> MAKRIATVSQTLRIGYVSSLLYGLLPEIIYLFRQQNPEIHIELIE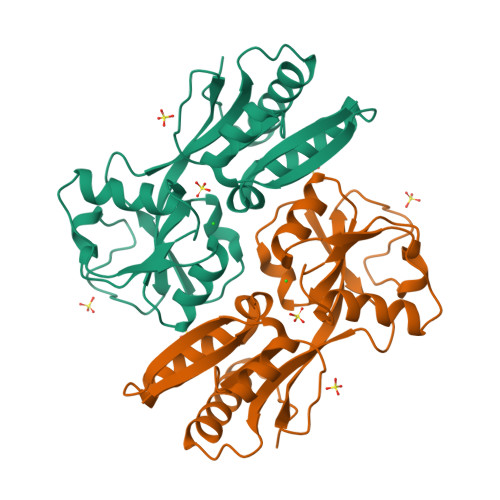CGTKDQINALKQGKIDLGFGRLKITDPAIRRIVLHKEQLKLAIHKHHHPNQFAATGVHLSQIIDEPMLLYPVSQKPNFATFIQSLFTELGLVPSKLTEIREIQLALGLVAAGEGVCIVPASAMDIGVKNLLYIPILDDDAYSPISLAVRNMDHSNYIPKILACVQEVFATHHIRPLIESILEHHHHHH> KA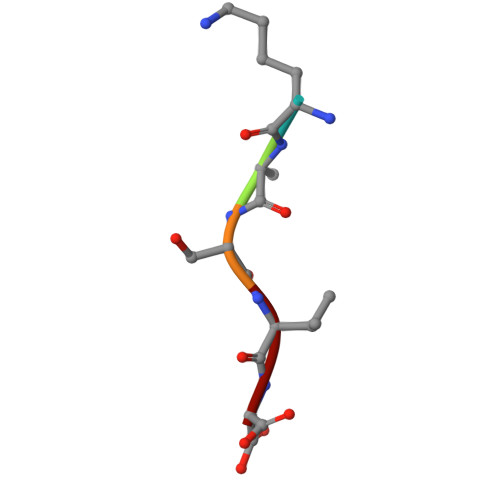SVG2-(4-methylphenyl)-3-(pyridin-2-ylmethoxy)pyridine | C18 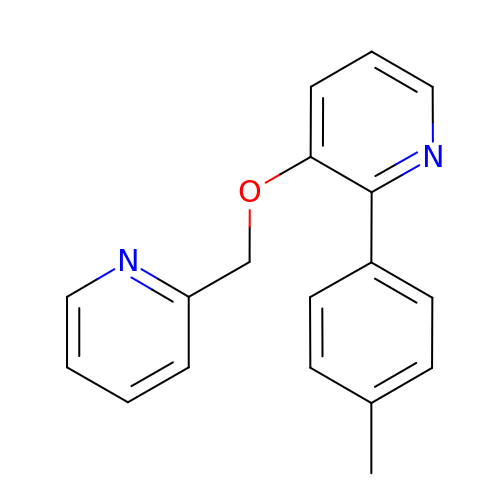H16 N2 O | GEICNUUKZLWKET-UHFFFAOYSA-N> DGVRIFNSLAATVYADSTAAHADMQGRRLKAVSDGLDHNGTGLRVIAQTQQDGGTWEQGGVEGKMRGSTQ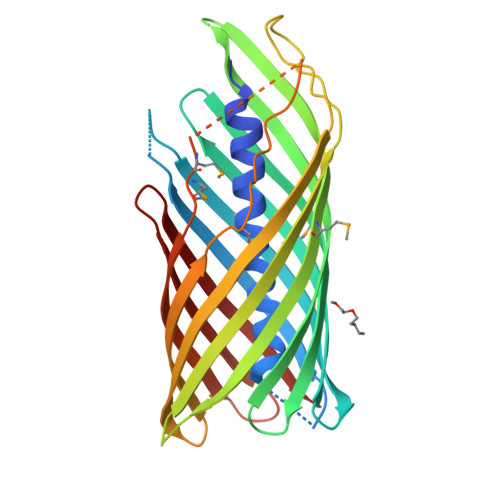TVGIAAKTGENTTAAATLGMGRSTWSENSANAKTDSISLFAGIRHDAGDIGYLKGLFSYGRYKNSISRSTGADEHAEGSVNGTLMQLGALGGVNVPFAATGDLTVEGGLRYDLLKQDAFAEKGSALGWSGNSLTEGTLVGLAGLKLSQPLSDKAVLFATAGVERDLNGRDYTVTGGFTGATAATGKTGARNMPHTRLVAGLGADVEFGNGWNGLARYSYAGSKQYGNHSGRVGVGYRF> MFEFTLMVVGESGLGKSTLINSLFLTDLYPERVIPGAAEKIERTVQIEASTVEIEERGVKLRLTVVDTPGYGDAINCRDCFKTIISYIDEQFERYLHDESGLNRRHIIDNRVHCCFYFISPFGHGLKPLDVAFMKAIHNKVNIVPVIAK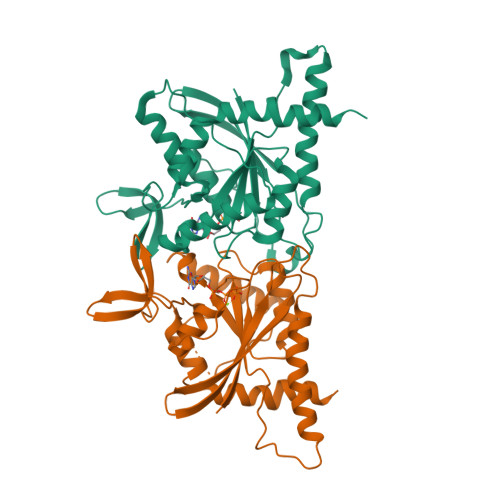ADTLTLKERERLKKRILDEIEEHNIKIYHLPDAESDEDEDFKEQTRLLKASIPFSVVGSNQLIEAKGKKVRGRLYPWGVVEVENPEHNDFLKLRTMLITHMQDLQEVTQDLHYENFRSERLKRGG;> MGSSHHHHHHSQDPNSSSARLQVDKLFCFNILCVGETGIGKSTLMDTLFNTKFESDPATHNEPGVRLKARSYELQESNVRLKLTIVDTVGFGDQINKDDSYKPIVEYIDAQFEAYLQEELKIKRSLFNYHDTRIHACLYFIAPTGHSLKSLDLVTMKKLDSKVNIIPIIAKADTIAKNELHKFKSKIMSELVSNGVQIYQFPTDEETVAEINATMSVHLPFAVVGSTEEVKIGNKMAKARQYPWGVVQVENENHCDFVKLREMLIRVNMEDLREQTHTRHYELYRRCKLEEMG2-[[1-ethoxy-7-[4-(3-fluoranyl-5-methoxy-phenyl)carbonyl-2,6-dimethyl-phenoxy]-4-oxidanyl-isoquinolin-3-yl]carbonylamino]ethanoic 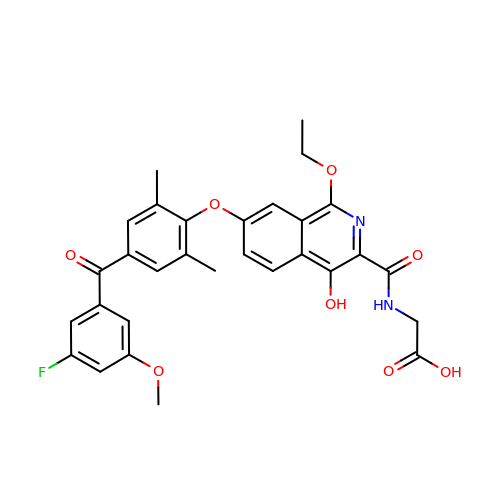acid | C30 H27 F N2 O8 | DLRMKPITDQZMBN-UHFFFAOYSA-N>[8x]MQEKDASSQGFLPHFQHFATQAIHVGQDPEQWTSRAVVPPISLSTTFKQGAPGQHSGFTYSRSGNPTRNCLEKAVAALDGAKYCLAFASGLAATVTITHLLKAGDQ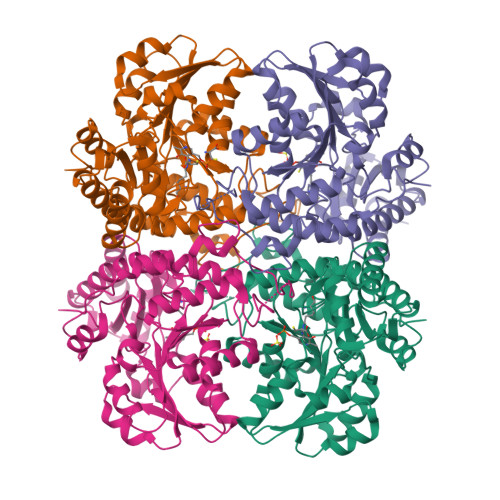IICMDDVYGGTNRYFRQVASEFGLKISFVDCSKIKLLEAAITPETKLVWIETPTNPTQKVIDIEGCAHIVHKHGDIILVVDNTFMSPYFQRPLALGADISMYSATKYMNGHSDVVMGLVSVNCESLHNRLRFLQNSLGAVPSPIDCYLCNRGLKTLHVRMEKHFKNGMAVAQFLESNPWVEKVIYPGLPSHPQHELVKRQCTGCTGMVTFYIKGTLQHAEIFLKNLKLFTLAVSLGGFESLAELPAIMTHASVLKNDRDVLGISDTLIRLSVGLEDEEDLLEDLDQALKAAHPPSGSHS> MNEKYEAVIGLEIHVQMDTKTKMFCGCKVEFGAEPNTNVCPVCLGMPGALPIVNKRAVEYAIRASLALNCEVHEESVFARKHYFYPDLPKGYQISQYEKPLATNGWVELNLPNGEKKKVRIRRLHIEEDAGKNIHEGDKTLVDLNRAGTPLMEIVTEPDIRTPEEARLFLEKLRNIMRYAGVSKADMEKGQLRCDINVSIRPKGSKEFGTRVEIKNVNSFRFVQKALEYEIERQINVVEEGGEVVQETRTFDPQTGKTYPMRTKEEAEDYRYFPDPDLVPLKVKKEWIEEIKKNMPELPDQRFERLIKEYGLSEYE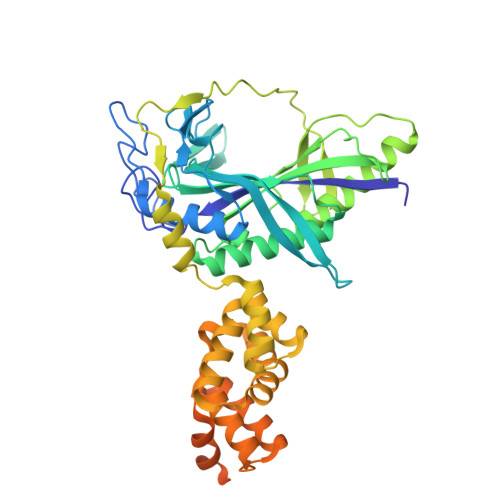AGILVNHKEVGDFFEEAVRHFKEPKGIVNWLINDLLGLLRDKGISIEESPVKPEHLAELVKLIKEKVISTKIGKEVIKEMVETGKTPSQIVEEKGLKQITDENQIKELVKKIFEKHPKEVERLKQGEEKLIGFFVGQVMRETRGKANPQVVNKVIRELVKEV> GTCGGCCCAC;> GUGG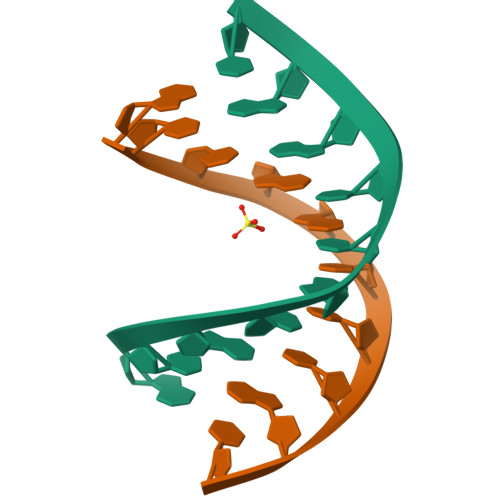GCCGAC>[2x]GNTDYDWKQFEQNSKYEQGYQKSHPTIQLFWKAFH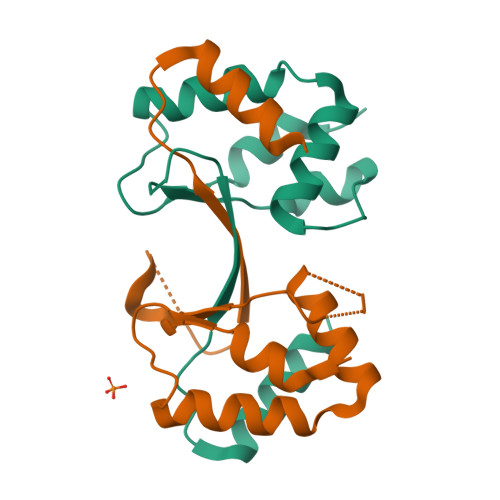KLTLDEKKKFLFFLTGRDRLHARGIQKMEIVFRSPETFSERDHPTSITCHNILSLPKYSTMERMEEALQVAINNNRGFVSPMLTQS> MSK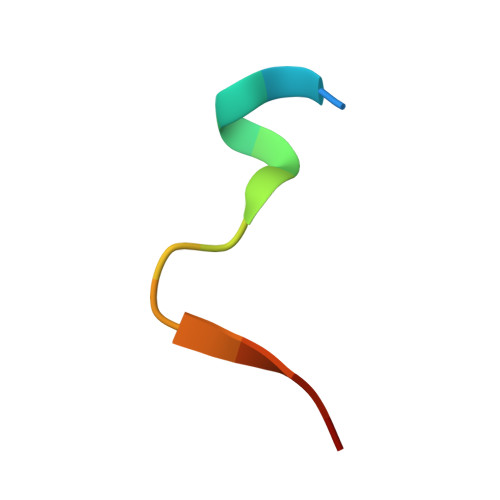FLDRFRYFKQKG> MESKVVVPAQGKKITLQNGKLNVPENPIIPYIEGDGIGVDVTPAMLKVVDAAVEKAYKGERKISWMEIYTGEKSTQVYGQDVWLPAETLDLIREYRVAIKGPLTTPVGGGIRELLVALRQELDLYICLRPVRYYQGTPSPVKHPELTDMVIFRENSEDIYAGIEWKADSADAEKVIKFLREEMGVKKIRFPDHCGIGIKPCSEEGTKRLVRAAIEYAIANDRDSVTLVHKGNIMKFTEGAFKDWGYQLAREEFGGELIDGGPWLKVKNPNTGKEIVIKDVIADAFLQQILLRPAEYDVIACMNLNGDYISDALAAQVGGIGIAPGANIGDECALFEATHGTAPKYAGQDKVNPGSIILSAEMMLRHMGWTEAADLIVKGMEGAINA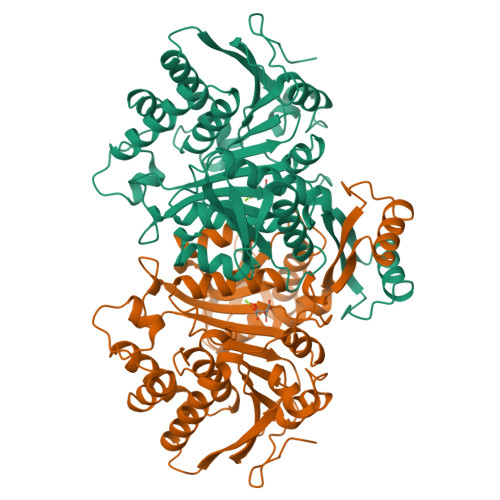KTVTYDFERLMDGAKLLKCSEFGDAIIENM2-(5-(benzyloxy)-1-hydroxy-1,3-dihydrobenzo[c][1,2]oxaborol-3-yl)acetic 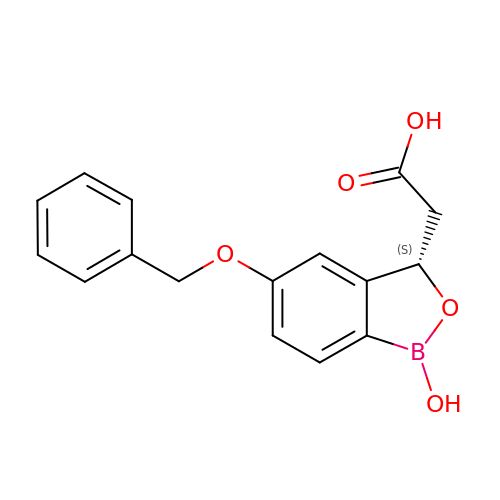acid | C16 H15 B O5 | HVZSXJPAWAMXTG-HNNXBMFYSA-N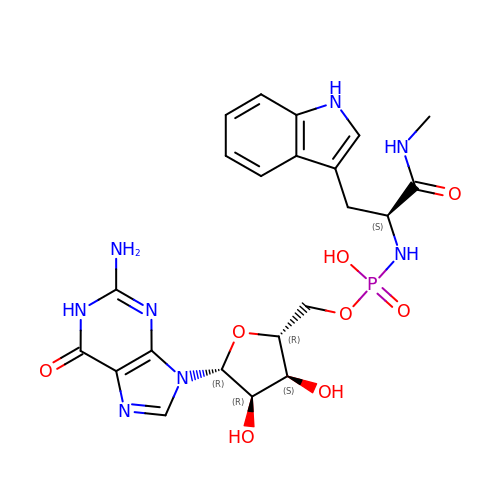[(2~{R},3~{S},4~{R},5~{R})-5-(2-azanyl-6-oxidanylidene-1~{H}-purin-9-yl)-3,4-bis(oxidanyl)oxolan-2-yl]methoxy-~{N}-[(2~{S})-3-(1~{H}-indol-3-yl)-1-(methylamino)-1-oxidanylidene-propan-2-yl]phosphonamidic acid | C22 H27 N8 O8 P | RVXFFUUVRZGQHL-QMBVYZDCSA-N In eukaryotic cells, newly synthesized proteins are transported from the endoplasmic reticulum (ER) to the Golgi apparatus through the action of the coat protein complex II (COPII). Sar1 recruits heterodimers of Sec23 and Sec24 to the membrane, thereby forming the inner layer of the COPII coat. Sec23/24 is an adaptor complex: Sec24 binds transport cargo while Sec23 interacts with Sar1 and recruits Sec13/31. Sec13/31 heterotetramers constitute the outer coat layer, thought to polymerise into cages that enclose the budding membrane.

We incubated giant unilamellar vesicles (GUVs) with yeast COPII proteins (Sec12, Sar1, Sec23/24, Sec13/31) in the presence of a non-hydrolysable GTP analogue GMP-PNP. To understand the architecture of the Sec13/31 outer coat we applied reference free, contrast-transfer function (CTF) corrected, subtomogram averaging to solve the 3D structure of the vertex, and of the connecting rods to resolutions of ∼40 Å (and ‘Materials and methods’). The connecting rods are consistent in shape and size with Sec13/31 heterotetramers, and are bent in the middle by approximately 15°. This same bend is seen in the solved X-ray crystal structure, which can be fitted into the densities as a rigid body. In contrast, there is a 45° bend in the rods of in vitro-assembled protein cages (Stagg et al., 2008). When we analysed the distribution of vertices and rods on the tubular membranes we found that they assembled regions of rhomboidal lattice.

>[2x]MVKLAEFSRTATFAWSHDKIPLLVSGTVSGTVDANFSTDSSLELWSLLAADSEKPIASLQVDSKFNDLDWSHNNKIIAGALDNGSLELYSTNEANNAINSMARFSNHSSSVKTVKFNAKQDNVLASGGNNGEIFIWDMNKCTESPSNYTPLTPGQSMSSVDEVISLAWNQSLAHVFASAGSSNFASIWDLKAKKEVIHLSYTSPNSGIKQQLSVVEWHPKNSTRVATATGSDNDPSILIWDLRNANTPLQTLNQGHQKGILSLDWCHQDEHLLLSSGRDNTVLLWNPESAEQLSQFPARGNWCFKTKFAPEAPDLFACASFDNKIEVQTLQNLTNTLDEQETETKQQESETDFWNNVSREESKEKPSVFHLQAPTWYGEPSPAAHWAFGGKLVQITPDGKGVSITNPKISGLESNTTLSEALKTKDFKPLINQRLVKVIDDVNEEDWNLLEKLSMDGTEEFLKEALAFDNDESDAQDDANNEKEDDGEEFFQQIETNFQPEGDFSLSGNIEQTISKNLVSGNIKSAVKNSLENDLLMEAMVIALDSNNERLKESVKNAYFAKYGSKSSLSRILYSISKREVDDLVENLDVSQWKFISKAIQNLYPNDIAQRNEMLIKLGDRLKENGHRQDSLTLYLAAGSLDKVASIWLSEFPDLEDKLKKDNKTIYEAHSECLTEFIERFTVFSNFINGSSTINNEQLIAKFLEFINLTTSTGNFELATEFLNSLPSDNEEVKTEKARVLIASGKSLPAQNPATATTSKAKYTNAKTNKNVPVLPTPGMPSTTSIPSMQAPFYGMTPGASANALPPKPYVPATTTSAPVHTEGKYAPPSQPSMASPFVNKTNSSTRLNSFAPPPNPYATATVPATNVSTTSIPQNTFAPIQPGMPIMGDYNAQSSSIPSQPPINAVSGQTPHLNRKANDGWNDLPLKVKEKPSRAKAVSVAPPNILSTPTPLNGIPANAASTMPPPPLSRAPSSVSMVSPPPLHKNSRVPSLVATSESPRASISNPYAPPQSSQQFPIGTISTANQTSNTAQVASSNPYAPPPQQRVATPLSGGVPPAPLPKASNPYAPTATTQPNGSSYPPTGPYTNNHTMTSPPPVFNKPPTGPPPISMKKRSNKLASIEQNPSQGATYPPTLSSSASPLQPSQPPTLASQVNTSAENVSHEIPADQQPIVDFLKEELARVTPLTPKEYSKQLKDCDKRLKILFYHLEKQDLLTQPTIDCLHDLVALMKEKKYKEAMVIHANIATNHAQEGGNWLTGVKRLIGIAEATLN;> VVIANAHNELIHDAVLDYYGKRLATCSSDKTIKIFEVEGETHKLIDTLTGHEGPVWRVDWAHPKFGTILASCSYDGKVLIWKEENGRWSQIAVHAVHSASVNSVQWAPHEYGPLLLVASSDGKVSVVEFKENGTTSPIIIDAHAIGVNSASWAPATIEEDGEHNGTKESRKFVTGGADNLVKIWKYNSDAQTYVLESTLEGHSDWVRDVAWSPTVLLRSYLASVSQDRTCIIWTQDNEQGPWKKTLLKEEKFPDVLWRASWSLSGNVLALSGGDNKVTLWKENLEGKWEPA;> VVIANAHNEMIHDAVMDYYGKRMATCSSDKTIKIFEVEGETHKLIDTLTGHEGPVWRVDWAHPKFGTILASCSYDGKVMIWKEENGRWSQIAVHAVHSASVNSVQWAPHEYGPMLLVASSDGKVSVVEFKENGTTSPIIIDAHAIGVNSASWAPATIEEDGEHNGTKESRKFVTGGADNLVKIWKYNSDAQTYVLESTLEGHSDWVRDVAWSPTVLLRSYMASVSQDRTCIIWTQDNEQGPWKKTLLKEEKFPDVLWRASWSLSGNVLALSGGDNKVTLWKENLEGKWEPA> AEQGPSLLQNKCMGCHIPEGNDTYSRISHQRKTPEGWLMSIARMQVMHGLQISDDDRRTLVKYLADKQGLAPSETDGVRYAMERRLNTVEQFDTQLSETCGRCHSGARVALQRRPAKEWEHLVNFHLGQWPSLEYQAQARDRDWLPIALQQVVPDLAKRYPLESAA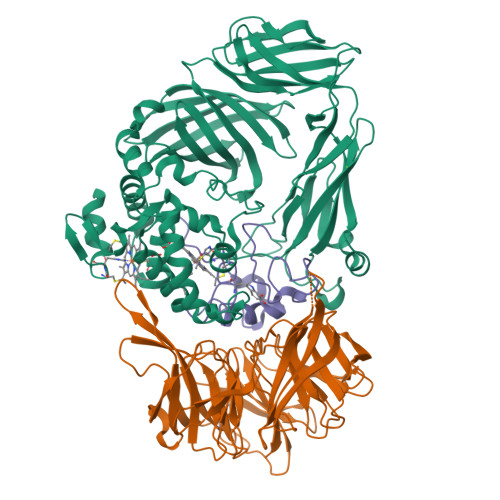WAEWQKARPKADALPGQWAFSGHMLAKGDVRGVMSVTPDQGDTFKVEVKGAYADGTPFNGSGSAILYNGYEWRGNVKVGDANLRQVFAALDGEMKGRMFEAEHDERGLDFTAVKEGKARLLAVQPAFIKAGGESEITLVGSGLAGKPDLGAGVEVTEVLEQTPTLVRLKARAAADAKPGQREVAVGTLKGVNLAVYDKVEEVKVVPAFSIARIGENGASVPKVQGRFEAEAWGKDANGQPLRIGYLPASWKVEPFNERAVEDEDVKFAGKMQADGVFVPGGAGPNPERKMMTNNAGNLKVIATLADGGQTGEGHMIVTVQRWNNPPLP;> ADTGPALKAGHEYMIVTNYPNNLHVVDVASDTVYKSCVMPDKFGPGTAMMAPDNRTAYVLNNHYGDIYGIDLDTCKNTFHANLSSVPGEVGRSMYSFAISPDGKEVYATVNPTQRLNDHYVVKPPRLEVFSTADGLEAKPVRTFPMPRQVYLMRAADDGSLYVAGPDIYKMDVKTGKYTVALPLRNWNRKGYSAPDVLYFWPHQSPRHEFSMLYTIARFKDDKQDPATADLLYGYLSVDLKTGKTHTQEFADLTELYFTGLRSPKDPNQIYGVLNRLAKYDLKQRKLIKAANLDHTYYCVAFDKKGDKLYLGGTFNDLAVFNPDTLEKVKNIKLPGGDMSTTTPQVFIR;> MSAVAGCTATTDPGWEVDAFGGVSSLCQPMEADLYGCSDPCWWPAQVPDMMSTYQDWNAQASNSAEDWRNLGTVFPKDK> GSHMASMKKKGSVVIVGRINLSGDTAYAQQTRGEEGCQETSQTGRDKNQVEGEVQIVSTATQTFLATSINGVLWTVYHGAGTRTIASPKGPVTQMYTNVDKDLVGWQAPQGSRSLTPCTCGSSDLYLVTRHADVIPVRRRGDSRGSLLSPRPISYLKGSAGGP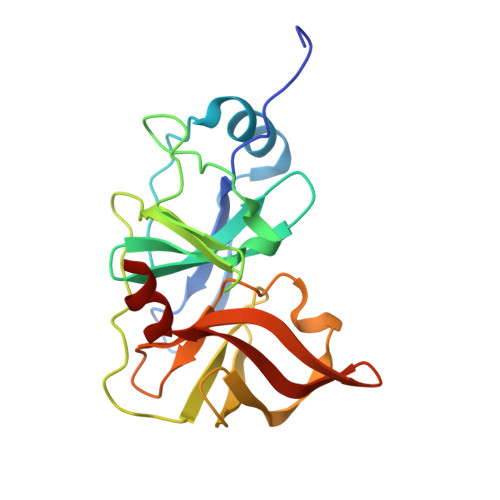LLCPAGHAVGIFRAAVSTRGVAKAVDFIPVESLETTMRSP> MFFTCGPNEAMVVSGFCRSPPVMVAGGRVFVLPCIQQIQRISLNTLTLNVKSEKVYTRHGVPISVTGIAQVKIQGQNKEMLAAACQMFLGKTEAEIAHIALETLEGHQRAIMAHMTVEEIYKDRQKFSEQVFKVASSDLVNMGISVVSYTLKDIHDDQDYLHSLGKARTAQVQKDARIGEAEAKRDAGIREAKAKQEKVSAQYLSEIEMAKAQRDYELKKAAYDIEVNTRRAQADLAYQLQVAKTKQQIEEQRVQVQVVERAQQVAVQEQEI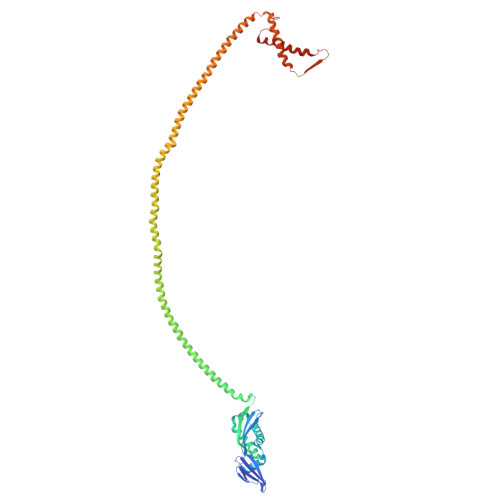ARREKELEARVRKPAEAERYKLERLAEAEKSQLIMQAEAEAASVRMRGEAEAFAIGARARAEAEQMAKKAEAFQLYQEAAQLDMLLEKLPQVAEEISGPLTSANKITLVSSGSGTMGAAKVTGEVLDILTRLPESVERLTGVSISQVNHK The highly expressed D7 protein family of mosquito saliva has previously been shown to act as an anti-inflammatory mediator by binding host biogenic amines and cysteinyl leukotrienes (CysLTs). In this study we demonstrate that AnSt-D7L1, a two-domain member of this group from Anopheles stephensi, retains the CysLT binding function seen in the homolog AeD7 from Aedes aegypti but has lost the ability to bind biogenic amines. Unlike any previously characterized members of the D7 family, AnSt-D7L1 has acquired the important function of binding thromboxane A2 (TXA2) and its analogs with high affinity. The crystal structure of AnSt-D7L1 contains two OBP-like domains and has a structure similar to AeD7.

The ligand-free form of the protein crystallized in the space group P212121 with one protein molecule in the asymmetric unit. The structure revealed two OBP domains with the N-terminal domain containing three disulfide bonds and the C-terminal domain containing two. In its overall structure, the protein is similar to AeD7 with an RMS deviation of 1.82 Å over 239 Cα positions. In AnSt-D7L1 the C-terminal domain also contains seven α-helices and is less similar in overall structure to AeD7 than is the N-terminal domain. In AnSt-D7L1, the second α-helix of AeD7 (B2) is not present. Rather, this region forms a predominantly coil structure extending between Lys 169 and Ser 184 containing a β-turn between residues Trp 173 and Gly 176. Arg 177 in AnSt-D7L1 is equivalent to Arg 176 in AeD7 but is positioned such that its side chain partially occupies the same space as the ligand in the AeD7-norepinephrine complex. Along with other changes, including the presence of tryptophan rather than leucine at position 173 in AnSt-D7L1, this modification acts to further fill the space equivalent to the biogenic amine binding pocket of the AeD7 C-terminal domain. Most notably, a histidine residue (position 189 in AeD7) that forms hydrogen bonds with the phenolic hydroxyl groups of serotonin and norepinephine is mutated to alanine (Ala 190) in AnSt-D7L1. In the absence of ligands, the segment between Leu 291 and the C-terminus (Phe 297) extends away from the surface of the protein and forms a β-turn between Thr 293 and His 296.

> QPWKALDAEQALYVYKRCYEDHLPSGSDRKTYMTLWNAWRLEPNDAITHCYAKCVLTGLQIYDPQENAFKSDRIPVQYQAYKTITQSKQKEVTEYQKALAAANAKSGSCVDLYNAYLPVHNRFVNLSRQLYHGTVEGAAKIYAAMPEIKQKGESFHAYCEKRAWKGNKQSEWKNGRRYKLTGSPELKDAIDCIFRGLRYMDDTGLKVDEIVRDFNLINKSELEPEVRSVLASCKGSEAYDYYVCLVNSRLKQHFKNAFDFHELRSADYAYLLRGKVYENPEKVKEEMKKLNTTVHF> QRTGRSALAVLIRACYRLQQQLQRTRRALLHHSDAVLT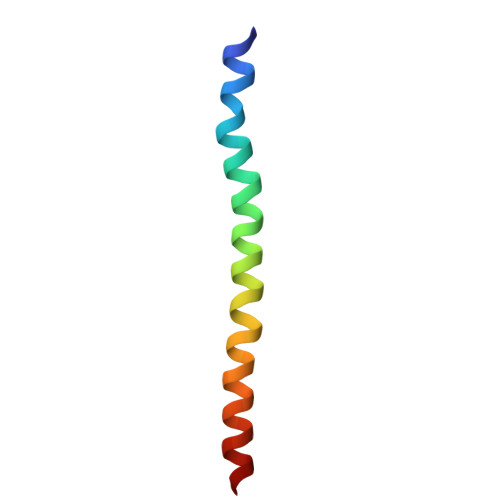SLHHVRMLL>[2x]GEFNTIQQLMMILNSASDQPSE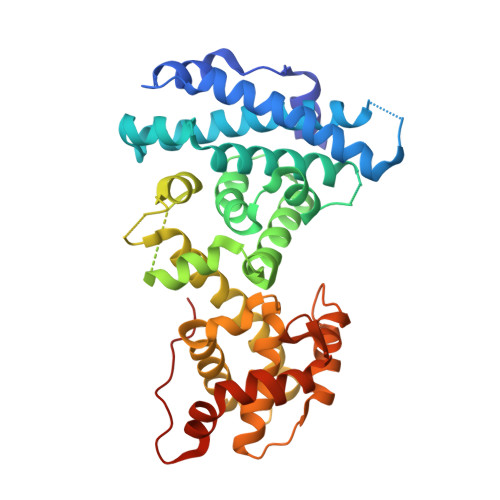NLISYFNNCTVNPKESILKRVKDIGYIFKEKFAKAVGQGCVEIGSQRYKLGVRLYYRVMESMLKSEEERLSIQNFSKLLNDNIFHMSLLACALEVVMATYSRSTSQNLDSGTDLSFPWILNVLNLKAFDFYKVIESFIKAEGNLTREMIKHLERCEHRIMESLAWLSDSPLFDLIKQSKDREGPTDHLESACPLNLPLQNNHTAADMYLEPVRAPKKKSTSLSLFYKKVYRLAYLRLNTLCERLLSEHPELEHIIWTLFQHTLQNEYELMRDRHLDQIVMCSMYGICKVKNIDLKFKIIVTAYKDLPHAVQETFKRVLIKEEEYDSIIVFYNSVFMQRLKTNILQYASTRPPTLAPIPHIPRSPYKFP In this study, we focus on chloride ion–pumping rhodopsin (ClR) from the marine flavobacterium Nonlabens marinus S1-08T. The conserved DTD motif (Asp85-Thr89-Asp96) of the bR family, residues 85, 89, and 96, is replaced by an NTQ motif (Asn98- Thr102-Gln109) in ClR. ClR structures at cryogenic and room temperatures clearly reveal an architecture composed of seven transmembrane helices (TM A to G). Cl− ions are transported from the extracellular (EC) side to the cytoplasmic (CP) side during each photocycle.

The torsion angle of C14-C15 = Nζ-Cε flips as a result from 155° (dark) to −65° (1 ps), and the retinal continues to change, showing a torsion angle of 187° at 2 ps and 126° at 100 ps. The distance between the Nζ atom and the centroid of the ionone ring increases from 12.7 Å (dark state) to 13.1 Å at 2 ps and then shrinks to about 12.2 Å as the retinal relaxes into the 13-cis configuration at 100 ps. The distance between Cl−1 and ND2 of Asn98 increases from 3.3 Å to 4.3 Å at 1 ps and then reduces to 3.7 Å at 2 ps as the sidechain rotates. TM-G kinks slightly at Lys235 on activation, with the angle between the two halves of TM-G increasing from about 4.6° in dark state to 4.8° at 1 ps and to 5.4° at 2 ps. At the 1 to 2 ps time points, the location of Cl– is close to Trp99, reflecting the dissociation from the PSB after photoactivation. The results also indicate that the structures at 1 to 2 ps time delays are mixtures of electronic excited state and the hot 13-cis state, while the structures at 50 to 100 ps correspond to the relaxed 13-cis state.

> KNIESLFDYSAGQFEFIDHLLTMGVGVHFAALIFFLVVSQFVAPKYRIATALSCIVMVSAGLILNSQAVMWTDAYAYVDGSYQLQDLTFSNGYRYVNWMATIPCLLLQLLIVLNLKGKELFSTATWLILAAWGMIITGYVGQLYEVDDIAQLMIWGAVSTAFFVVMNWIVGTKIFKNRATMLGGTDSTITKVFWLMMFAWTLYPIAYLVPAFMNNADGVVLRQLLFTIADISSKVIYGLMITYIAIQQSAAAGYVPAQQALGRI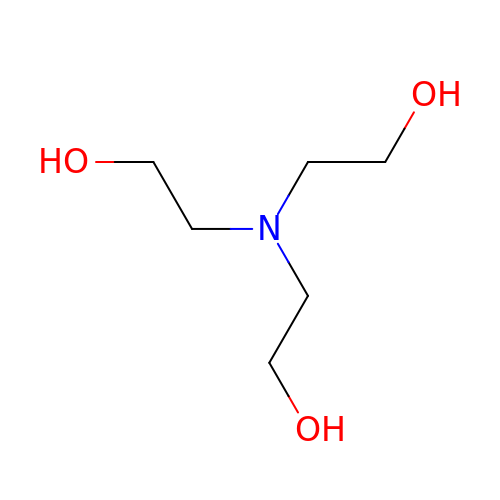2,2',2''-NITRILOTRIETHANOL | C6 H15 N O3 | GSEJCLTVZPLZKY-UHFFFAOYSA-N> MQT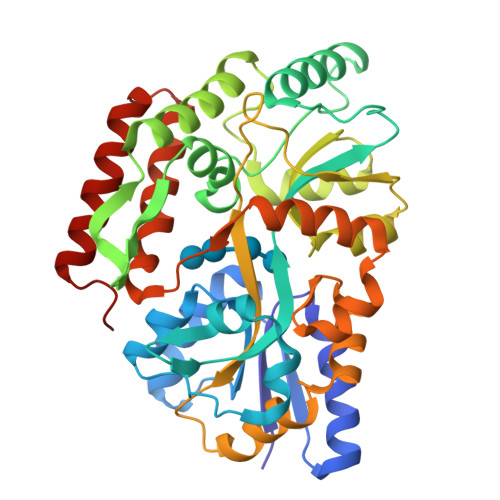KLTIWCSEKQVDILQKLGEEFKAKYGIPVEVQYVDFGSIKSKFLTAAPQGQGADIIVGAHDWVGELAVNGLIEPIPNFSDLKNFYDTALKAFSYGGKLYGVPYAMEAVALIYNKDYVDSVPKTMDELIEKAKQIDEEYGGEVRGFIYDVANFYFSAPFILGYGGYVFKETPQGLDVTDIGLANEGAVKGAKLIKRMIDEGVLTPGDNYGTMDSMFKEGLAAMIINGLWAIKSYKDAGINYGVAPIPELEPGVPAKPFVGVQGFMINAKSPNKVIAMEFLTNFIARKETMYKIYLADPRLPARKDVLELVKDNPDVVAFTQSASMGTPMPNVPEMAPVWSAMGDALSIIINGQASVEDALKEAVEKIKAQIEKGSHHHHHH> SPQPLEQIKLSESQLSGRVGMIEMDLASGRTLTAWRADERFPMMSTFKVVLCGAVLARVDAGDEQLERKIHYRQQDLVDYSPVSEKHLA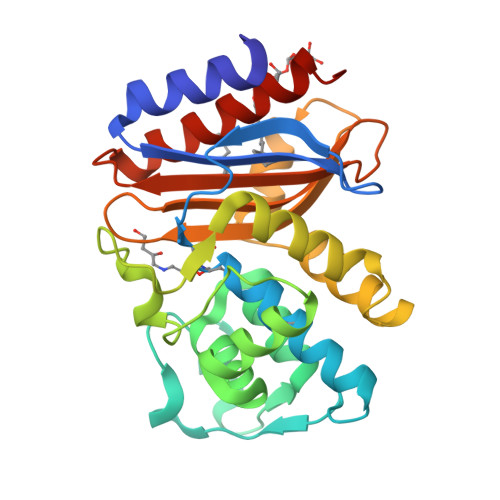DGMTVGELCAAAITMSDNSAANLLLATVGGPAGLTAFLRQIGDNVTRLDRWATELNEALPGDARDTTTPASMAATLRKLLTSQRLSARSQRQLLQWMVDDRVAGPLIRSVLPAGWFIADKTGAGERGARGIVALLGPNNKAERIVVIYLRDTPASMAERNQQIAGIGAALIEHWQRLMIL> MILDTDYITEDGKPVIRIFKKENGEFKIDYDRNFEPYIYALLKDDSAIEDVKKITAERHGTTVRVVRAEKVKKKFLGRPIEVWKLYFTHPQDVPAIRDKIKEHPAVVDIYEYDIPFAKRYLIDKGLIPMEGDEELKMLAFDIETLYHEGEEFAEGPILMISYADEEGARVITWKNIDLPYVDVVSTEKEMIKRFLKVVKEKDPDVLITYNGDNFAFAYLKKRSEKLGVKFILGREGSEPKIQRMGDRFAVEVKGRIHFDLYPVIRRTINLPTYTLEAVYEAIFGQPKEKVYAEEIAQAWETGEGLERVARYSMEDAKVTYELGKEFFPMEAQL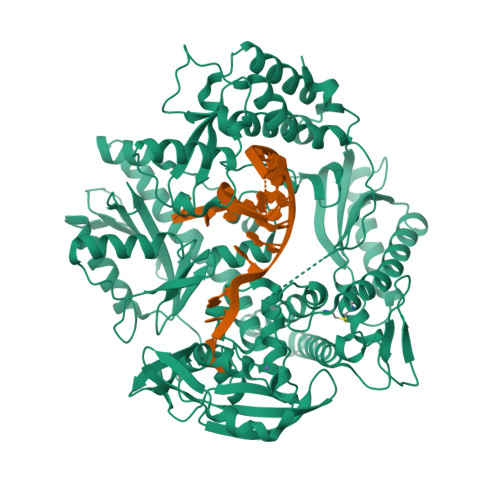SRLVGQSLWDVSRSSTGNLVEWFLLRKAYERNELAPNKPDERELARRRESYAGGYVKEPERGLWENIVYLDFRSLYPSIIITHNVSPDTLNREGCEEYDVAPQVGHKFCKDFPGFIPSLLGDLLEERQKVKKKMKATIDPIEKKLLDYRQRAIKILANSFYGYYGYAKARWYCKECAESVTAWGRQYIETTIREIEEKFGFKVLYADTDGFFATIPGADAETVKKKAKEFLDYINAKLPGLLELEYEGFYKRGFFVTKKKYAVIDEEDKITTRGLEIVRRDWSEIAKETQARVLEAILKHGDVEEAVRIVKEVTEKLSKYEVPPEKLVIYEQITRDLKDYKATGPHVAVAKRLAARGIKIRPGTVISYIVLKGSGRIGDRAIPFDEFDPAKHKYDAEYYIENQVLPAVERILRAFGYRKEDLRYQKTRQVGLGAWLKPKT> MGSSLRPLYMDVQATTPLDPRVLDAMLPYLINYYGNPHSRTHAYGWESEAAMERARQQVASLIGADPREIIFTSGATESNNIAIKGVARFYRSRKKHLITTQTEHKCVLDSCRSLEAEGFQVTYLPVQKSGIIDLKELEAAIQPDTSLVSVMTVNNEIGVKQPIAEIGRICSSRKVYFHTDAAQAVGKIPLDVNDMKIDLMSISGHKIYGPKGVGAIYIRRRPRVRVEALQSGGGQERGMRSGTVPTPLVVGLGAACEVAQQEMEYDHKRIS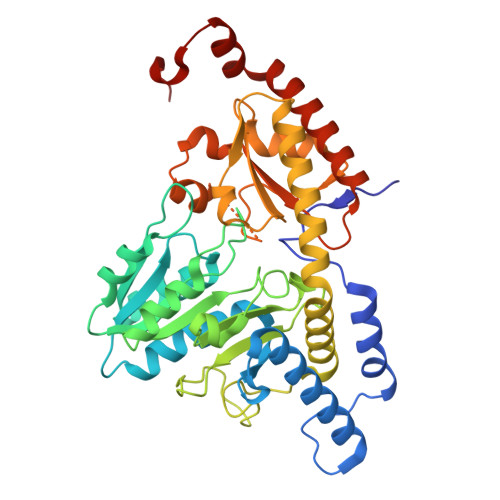KLSERLIQNIMKSLPDVVMNGDPKHHYPGCINLSFAYVEGESLLMALKDVALSSGSACTSASLEPSYVLRAIGTDEDLAHSSIRFGIGRFTTEEEVDYTVEKCIQHVKRLREMSPLWEMVQDGIDLKSIKWTQH5-(4-fluorophenyl)-2,3-dihydroxy-N-[(1-methylimidazol-4-yl)methyl]benzamide | C18 H16 F N3 O3 | 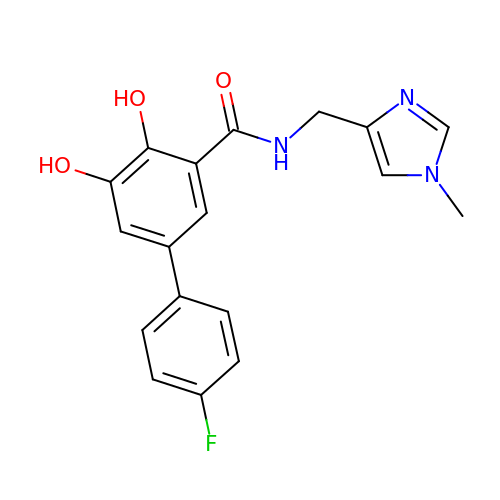ICFMTNZFOIXRGG-UHFFFAOYSA-N> XXXXXXXXXXXXXXXXXXXXXXXXXXXXXXXXXXXXXXXXXXXXXLERYRADLIDRKILRNKDHGVRAFAACCLSDILRLYAPDAPYTDKELTEIFRLFLAQLKLLQEPENGYLTQQTYLINNLLEYRSIVILTDLPSSSQLVEELFNIFYSPTNSTIQGNMFTAIGGILGEVISECDSLPMSALKMVFNKFLSHKRAESLDGINYKKDPGFEISLIICQTYSNRLGRHFIKFYSEIMYEVLGESDIHEKGIASSAYKTLVKIGNLTSELWKYAPELVGSVTGLLYQLLCSDNELFRESATKCVSKMLGTHSLINFAVAHSDTYKIWLSKMADISPHVRQAWVSEIPSILMSRSDLSDDISKGLAKALIDSDHTVRLSAIQTFHEVPVKRLWECLPNAAVFAGLVHLTRETRRDLRDECIDAVARIYTESIESIPKTNENKEIWGVVETIPSACFNLYYINDLEINMKVDLLTFEKFLPLGLSNEEFVQRLLTLLQGFNEKAFSSFYAFNRRQDQMSTVLWKFIEFCEETNSQSPAASLSDTKLIKTVEWISSGFPSHLNVEQILLAFRELN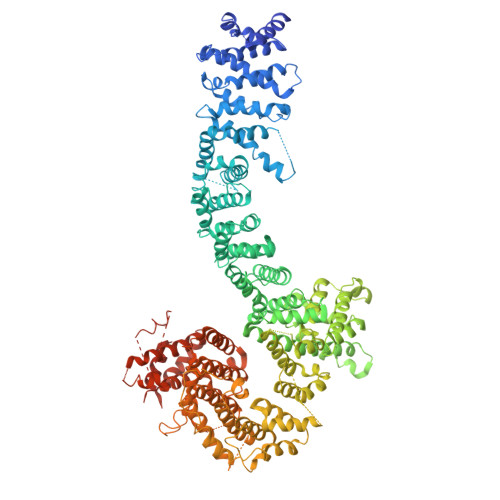DRRLYRLIKVAVAETSKHLTVRNAVSELFKRLEEPELFRKKNIKIESRFTRDNFSTVFRVLIYRAAPIIFNISNLPSFLNTSDSSNEDEKALKRQLIDNISIIKPGIFKDQVKNLVTIITEGETTGPGNTLSLAEAMRTVYKISKDKREHLDIEENTFFFQKLEDYAKEGNPLEAKYAIKLLGLAPNAAEYLSEVATAILPLDLKSKHFASNVLVLAEITKMQPQLLEKDSTEIVGLLIKDVLLSNDVVGDEDDQQAWFSDEDIYTGKADALSAKVFSLKLFANKIKVMAPDAHADEMTHAFTERTLKLFFYLVASGGELVSESNTDNYPTPANYQNKLRCCAGLHILKITKIASLSRFIKPQDISKLMNLVEDESLEVRSSFIGRLKDFLGDGSISIKFLPLVFFTAYEPDQALRTSTKMWINYTLSKENFRKGTFFERALPRLIHFIAHHPDVAEGLRLRETAFLTGLTTAIDYLVFYADSVLKASNLALLYYLAGRVRQYXXXXXXXXXXXXXXXXXXXXXXXXXXXXXXXXXXXXXXXXXXXXXXXXXXXXXXXXXX>ASMTGGQQMGRGSEFMGQSHTHDHHHDGYQAPPEDIALRVKALESLLIEKGLVDPAAMDLVVQTYEHKVGPRNGAKVVAKAWVDPAYKARLLADGTAGIAELGFSGVQGEDMVILENTPAVHNVFVCTLCSCYPWPTLGLPPAWYKAAPYRSRMVSDPRGVLAEFGLVIPANKEIRVWDTTAELRYMVLPERPAGTEAYSEEQLAELVTRDSMIGTGLPTQPTPSH[4x];>MNGIHDTGGAHGYGPVYREPNEPVFRYDWEKTVMSLLPALLANGNFNLDEFRHSIQRMGPAHYLEGTYYEHWLHVFENLLVEKGVLTATEVATGKAASGKTATPVLTPAIVDGLLSTGASAAREEGARARFAVGDKVRVLNKNPVGHTRMPRYTRGKVGTVVIDHGVFVTPDTAAHGKGEHPQHVYTVSFTSVELWGQDASSPKDTIRVDLWDDY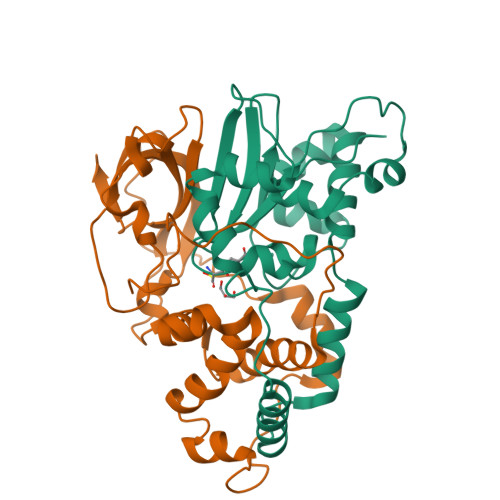LEPA[4x]>MGVEDEPLLRENPRRFVIFPIEYHDIWQMYKKAEASFWTAEAVDLSKDIQHWESLKPEERYFISHVLAFFAASDGIVNENLVERFSQEVQITEARCFYGFQIAMENIHSEMYSLLIDTYIKDPKEREFLFNAIETMPCVKKKADWALRWIGDKEATYGERVVAFAAVEGIFFSGSFASIFWLKKRGLMPGLTFSNELISRDEGLHCDFACLMFKHLVHKPSEERVREIIINAVRIEQEFL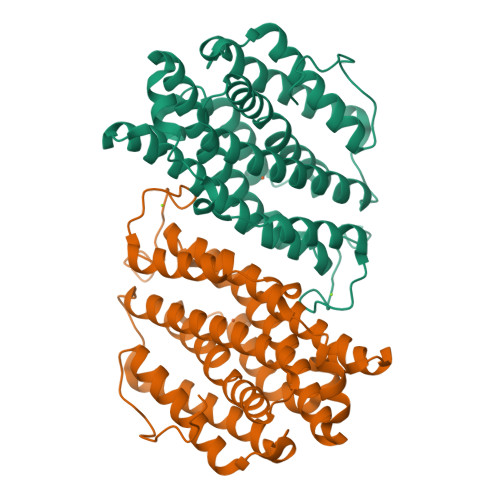TEALPVKLIGMNCTLMKQYIEFVADRLMLELGFSKVFRVENPFDFM[2x]> MDTTVPTFSLAELQQGLHQDEFRRCLRDKGLFYLTDCGLTDTELKSAKDIVIDFFEHGSEAEKRAVTSPVPTMRRGFTGLESESTAQITNTGSYSDYSMCYSMGTADNLFPSGDFERIWTQYFDRQYTASRAVAREVLRATGTEPDGGVEAFLDCEPLLRFRYFPQVPEHRSAEEQPLRMAPHYDLSMVTLIQQTPCANGFVSLQAEVGGAFTDLPYRPDAVLVFCGAIATLVTGGQVKAPRHHVAAPRRDQIAGSSQTSSVFFLRPNADFTFSVPLARE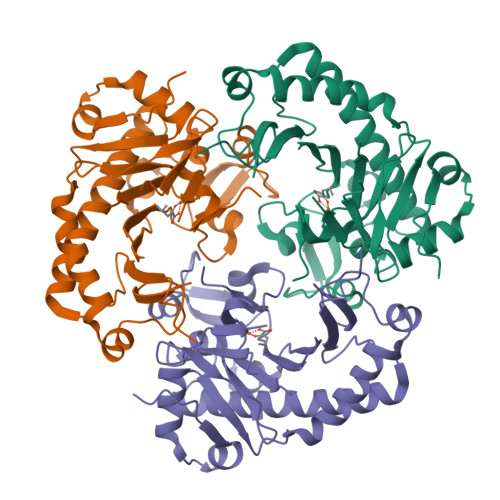CGFDVSLDGETATFQDWIGGNYVNIRRTSKA>MTAQTPIHVYSEIGKLKKVLLHRPGKEIENLMPDYLERLLFDDIPFLEDAQKEHDAFAQALRDEGIEVLYLETLAAESLVTPEIREAFIDEYLSEANIRGRATKKAIRELLMAIEDNQELIEKTMAGV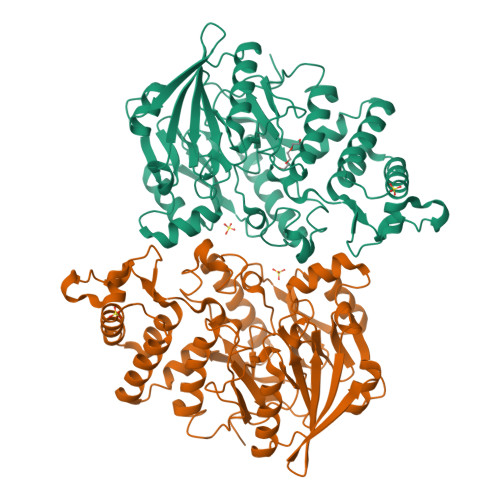QKSELPEIPASEKGLTDLVESNYPFAIDPMPNLYFTRDPFATIGTGVSLNHMFSETRNRETLYGKYIFTHHPIYGGGKVPMVYDRNETTRIEGGDELVLSKDVLAVGISQRTDAASIEKLLVNIFKQNLGFKKVLAFEFANNRKFMHLDTVFTMVDYDKFTIHPEIEGDLRVYSVTYDNEELHIVEEKGDLAELLAANLGVEKVDLIRCGGDNLVAAGREQWNDGSNTLTIAPGVVVVYNRNTITNAILESKGLKLIKIHGSELVRGRGGPRCMSMPFEREDI[8x]>MTIKTKAELLNKWKPLLEGEGLPEIANSKQAIIAKIFENQEKDFQTAPEYKDEKIAQAFGSFLTEAEIGGDHGYNATNIAAGQTSGAVTQIGPAVMGMVRRAIPNLIAFDICGVQPMNSPTGQVFALRAVYGKDPVAAGAKEAFHPMYGPDAMFSGQGAAKKFPALAASTQTTVGDIYTHFFQETGTVYLQASVQVTIDAGATDAAKLDAEIKKQMEAGALVEIAEGMATSIAELQEGFNGSTDNPWNEMGFRIDKQVIEAKSRQLKAAYSIELAQDLRAVHGMDADAE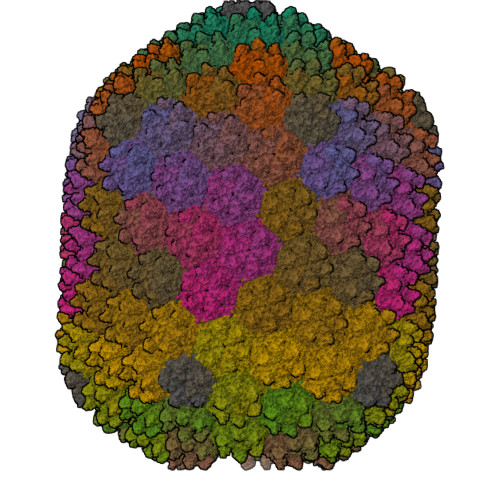LSGILATEIMLEINREVVDWINYSAQVGKSGMTLTPGSKAGVFDFQDPIDIRGARWAGESFKALLFQIDKEAVEIARQTGRGEGNFIIASRNVVNVLASVDTGISYAAQGLATGFSTDTTKSVFAGVLGGKYRVYIDQYAKQDYFTVGYKGPNEMDAGIYYAPYVALTPLRGSDPKNFQPVMGFKTRYGIGINPFAESAAQAPASRIQSGMPSILNSLGKNAYFRRVYVKGI[180x];>MAKINELLRESTTTNSNSIGRPNLVALTRATTKLIYSDIVATQRTNQPVAAFYGIKYLNPDNEFTFKTGATYAGEAGYVDREQITELTEESKLTLNKGDLFKYNNIVYKVLEDTPFATIEESDLELALQIAIVLLKVRLFSDAASTSKFESSDSEIADARFQINKWQTAVKSRKLKTGITVELAQDLEANGFDAPNFLEDLLATEMADEINKDILQSLITVSKRYKVTGITDSGFIDLSYASAPEAGRSLYRMVCEMVSHIQKESTYTATFCVASARAAAILAASGWLKHKPEDDKYLSQNAYGFLANGLPLYCDTNSPLDYVIVGVVENIGEKEIVGSIFYAPYTEGLDLDDPEHVGAFKVVVDPESLQPSIGLLVRYALSANPYTVAKDEKEARIIDGGDMDKMAGRSDLSVLLGVKLPKIIIDE[11x]1-deoxy-1-[8-(dimethylamino)-7-methyl-2,4-dioxo-3,4-dihydrobenzo[g]pteridin-10(2H)-yl]-D-ribitol | C18 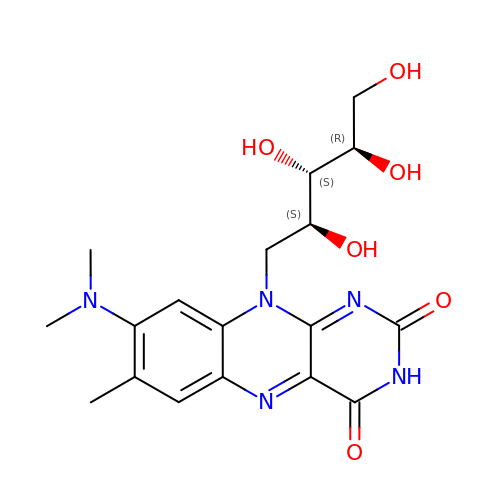H23 N5 O6 | IGQLDUYTWDABFK-GUTXKFCHSA-N>MKQYLELMQKVLDEGTQKNDRTGTGTLSIFGHQMRFNLQDGFPLVTTKRCHLRSIIHELLWFLQGDTNIAYLHENNVTIWDEWADENGDLGPVYGKQWR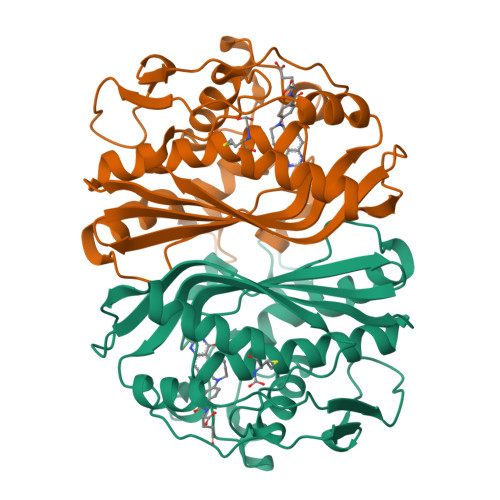AWPTPDGRHIDQITTVLNQLKNDPDSRRIIVSAWNVGELDKMALAPCHAFFQFYVADGKLSCQLYQQSCDVFLGLPFNIASYALLVHMMAQQCDLEVGDFVWTGGDTHLYSNHMDQTHLQLSREPRPLPKLIIKRKPESIFDYRFEDFEIEGYDPHPGIKAPVAI[2x]>[2x]DAVVAPISVPENGKGPFPQRLNQLKSNKDRDTKIFYSITGPGADSPPEGVFAVEKETGWLLLNKPLDREEIA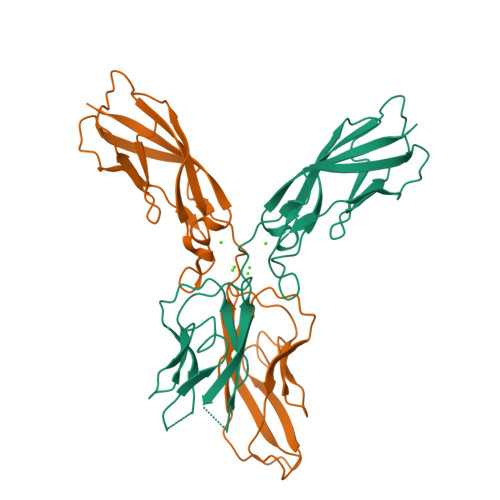KYELFGHAVSENGASVEDPMNISIIVTDQNDHKPKFTQDTFRGSVLEGVLPGTSVMQVTATDEDDAIYTYNGVVAYSIHSQEPKDPHDLMFTIHRSTGTISVISSGLDREKVPEYTLTIQATDMDGDGSTTTAVAVVEILD>[2x]MPELPEVETTLRGIAPHIEGKTVEAVVLRQLKLRWQ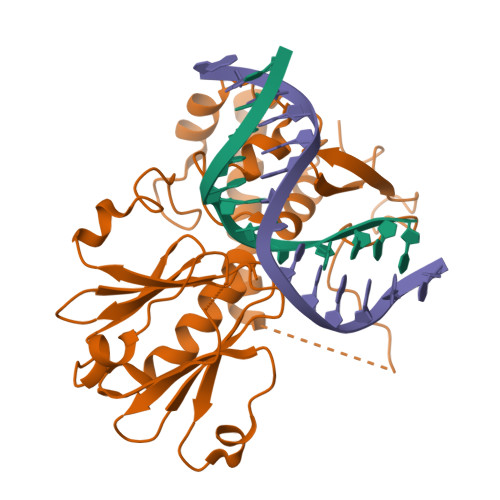INPDLGEILSGRQVLSCGRRAKYLLIRFQTGVLLIHLGMSGSLRIFTPSDGRIGRPDRHDHVDIVFSDGTVMRYRDPRKFGAILWYEGIEEHHPLLEKLGPEPLSEAFCADYLYARLKAQKRAVKLALMDNAVVVGVGNIYANESLFRAGISPHRPANRLKKKECALLVETVKAVLQRAIETGGSTLRDFVDSDGKSGYFQQEYTVYGRHNQPCPRCGGLVVKETLGQRGTFYCPNCQK>SNAMNLNQLDIIVSNVPQVCADLEHILDKKADYANDGFAQFTIGSHCLMLSQNHLVPLENFQSGIII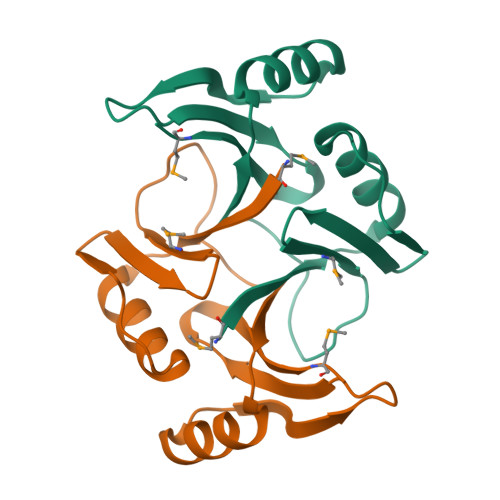HIEVEDVDQNYKRLNELGIKVLHGPTVTDWGTESLLVQGPAGLVLDFYRMK[2x]>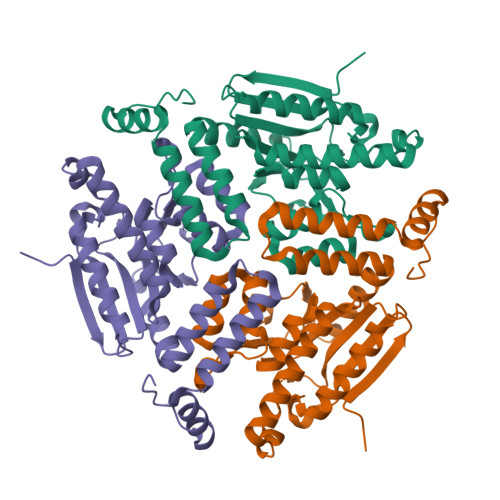 GHMPEFKVDARGPIEIWTIDGESRRNAISRAMLKELGELVTRVSSSRDVRAVVITGAGDKAFCAGADLKERATMAEDEVRAFLDGLRRTFRAIEKSDCVFIAAINGAALGGGTELALACDLRVAAPAAELGLTEVKLGIIPGGGGTQRLARLVGPGRAKDLILTARRINAAEAFSVGLANRLAPEGHLLAVAYGLAESVVENAPIAVATAKHAIDEGTGLELDDALALELRKYEEILKTEDRLEGLRAFAEKRAPVYKGR>ADSDINIKTGTTDIGSNTTVKTGDLVTYDKENGMHKKVFYSFIDDKNHNKKLLVIRTKGTIAGQYRVYSEEGANKSGLAWPSAFKVQLQLPDNE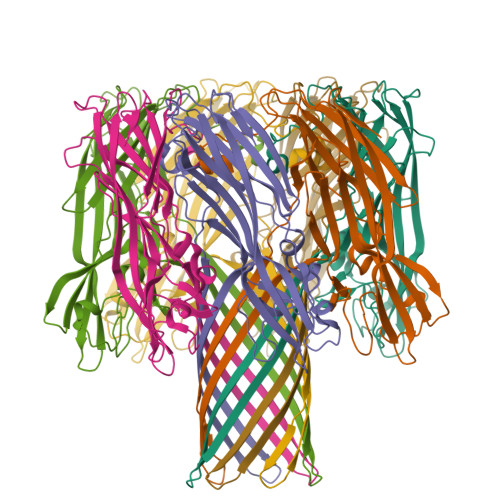VAQISDYYPRNSIDTKEYNSTLTYGFNGNVTGDDTGKIGGLIGANVSIGHTLKYVQPDFKTILESPTDKKVGWKVIFNNMVNQNWGPYDRDSWNPVYGNQLFMKTRNGSMKAADNFLDPNKASSLLSSGFSPDFATVITMDRKASKQQTNIDVIYERVRDDYQLHWTSTNWKGTNTKDKWTDRSSERYKIDWEKEEMTN[7x]>[5x]AKITKVQVGEALVGDGNEVAHIDLIIGPRGSPAETAFCNGLVNNKHGFTSLLAVIAPNLPCKPNTLMFNKVTINDARQAVQMFGPAQHGVAMAVQDAVAEGIIPADEADD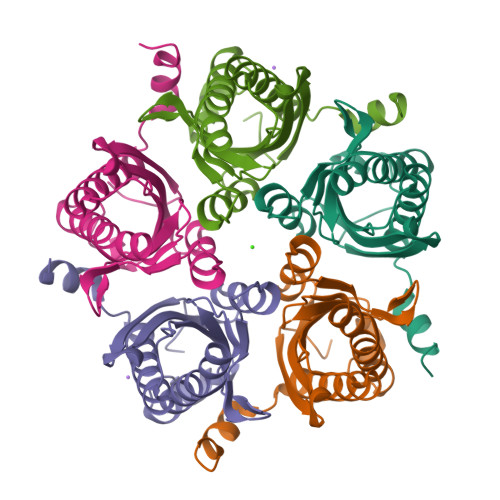LYVLVGVFIHWEAADDAKIQKYNYEATKLSIQRAVNGEPKASVVTEQRKSATHPFAANA N-{(1S,2R)-1-benzyl-2-hydroxy-3-[(3-methoxybenzyl)amino]propyl}-7-ethyl-1-methyl-3,4-dihydro-1H-[1,2,5]thiadiazepino[3,4,5-hi]indole-9-carboxamide 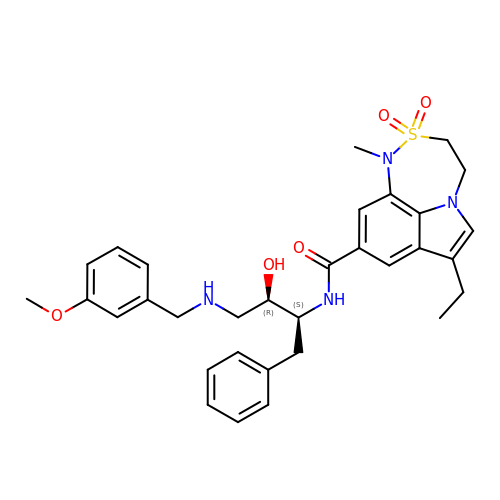2,2-dioxide | C32 H38 N4 O5 S | MNGUVHPNHVMEDL-MFMCTBQISA-N(6~{S},9~{a}~{S})-6-(3-azidopropyl)-8-(naphthalen-1-ylmethyl)-4,7-bis(oxidanylidene)-~{N}-[4,4,4-tris(fluoranyl)butyl]-3,6,9,9~{a}-tetrahydro-2~{H}-pyrazino[1,2-a]pyrimidine-1-carboxamide 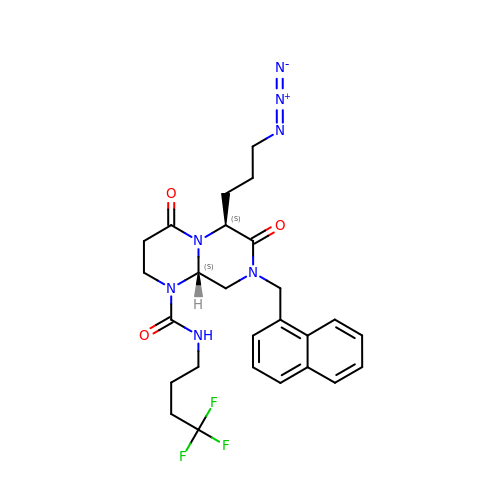| C26 H30 F3 N7 O3 | JEFJDQXONGAAEJ-FCHUYYIVSA-N>GMNPYERGPNPTDALLEARSGPFSVSEENVSRLSASGFGGGTIYYPRENNTYGAVAISPGYTGTEASIAWLGERIASHGFVVITIDTITTLDQPDSRAEQLNAALNHMINRASSTVRSRIDSSRLAVMGHAMGGGGSLRLASQRPDLKAAIPLTPWHLNKNWSSVTVPTLIIGADLDTIAPVATSAKPIYNSLPSSISKAYLELDGATHFAPNIPNKIIGKYSVAWLKRFVDNDTRYTQFLCPGPRDGLFGEVEEYRSTCPF[2x]

Cutinase is an esterase that belongs to the α/β-hydrolase superfamily and primarily hydrolyzes cutin from plants. Unlike lipases, cutinases lack the active site-covering lid structure such that the substrate-binding cleft is exposed and directly accessible from bulk solution. In addition, the substrate-binding site is more expansive in cutinases compared to esterases, benefiting the binding of bulkier macromolecules. In this work, we investigate the PBAT hydrolysis potency of cutinases and PET-degrading enzymes, and find that cutinases outcompete other reported enzymes.

We further constructed the inactive variant S170A to obtain a complex structure of BTa but failed to obtain any dataset that contains additional electron density that can be modeled with the ligand. We thus turned to a BTa-like compound MHET, which is composed of TPA and ethylene glycol linked via an ester bond. As a result, the structure of the S170A variant was determined in apo- and MHET-bound forms to 2.21 and 1.82 Å resolutions, respectively. In the MHET-bound complex, the omit map clearly indicates the location of MHET in the active site. Notably, the ethylene glycol portion of the bound MHET was located outwards and away from the catalytic center, opposing the direction of those in other MHET complexes (see below). Nevertheless, the hydroxyl group of S170 is estimated at 2.9 Å from the carbonyl carbon of MHET, which is within range for nucleophilic attack. Therefore, the complex structure should present the substrate-binding mode of TfCut-DM. The residues that ineract with MHET, Y100, M171, W195, and I218, are conserved in IsPETase and LCC-ICCG, while I218 has an alternative residue in LCC-ICCG. Superimposing the MHET-bound complex of IsPETase and TfCut-DM indicates that the ligand binding modes are similar. In both complexes, the TPA residue of MHET is bound to the TPA-interacting Trp (W195 in TfCut-DM) that adopts B-type conformation via a T-stacking force.> MAEQAVPYGRKTQHTPALKEVHILWITAGLGCDGDSVSITAASQPSVEDVVLGAIPGLPKVHLHNPVLAYENGDEFMAPFHKAARGEIDNFVLV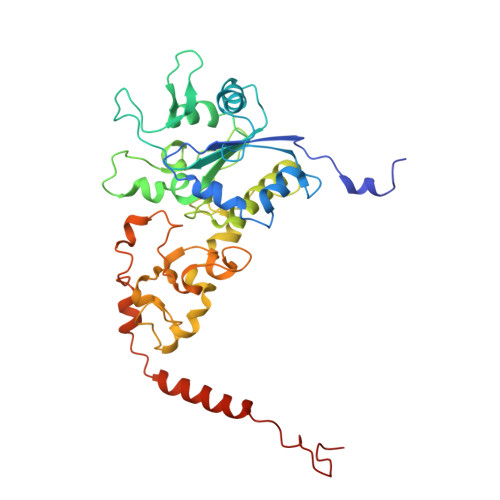LEGSIPNERINGEGYWAAMGTDPQTHQPITIPEWLDRLAPKALAVVGAGTCATYGGIHAMEGNPTGCMGLADYLGWQWKSRAGLPIVNVPGCPVQPDNFMETLLYLLYQLAGLAPMIPLDEALRPKWLFTRTVHDGCDRAGSYEQAIFATEYGNPNCIVKLGCWGPVVQCNVPKRGWIAGVGGCPNVGGICIGCTMPGFPDKFMPFMDAPPGAVLSSNLIKSYGPLIRSLRKLTKDTLNDEPKWRHNQPVLTTGYRG>[2x]GSHMDLTSIQWRMPEWVQSMGGLRTENVLEYFSQSPFYSH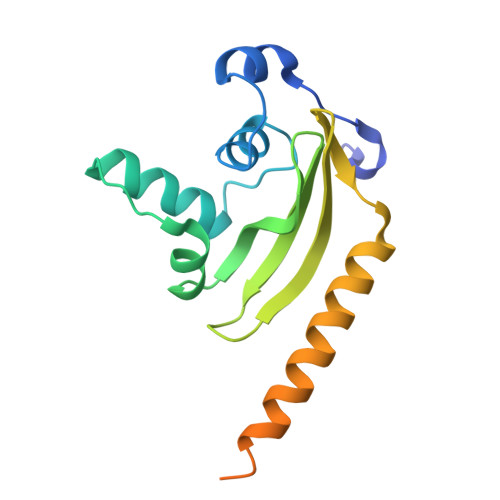KSNNEMLKMQSQFNALDLGDLNSQLKRLTGIQFVIIHERPPFLWVIQKQNRLNENEVKPLTVYFVCNENIYMAPNAYTLLATRMLNATYCFQKALTKIEKFPQYNPQEGYTYPKLSNDNLEVDHSNTNEPADENK>[4x]MATNGMRPIHPGEILRDEFLMEFDISPAALARALKV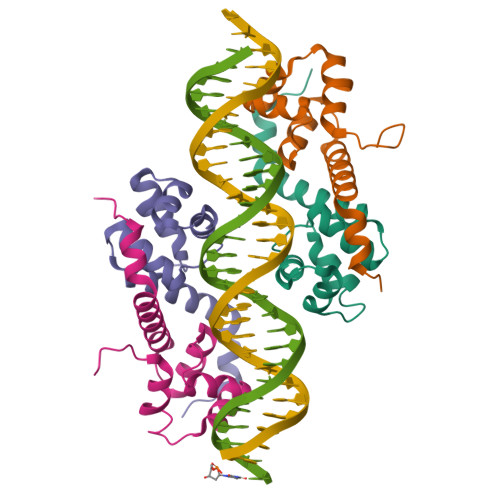SAPTVNDIVREQRGISADMAIRLGRYFDTSAQFWMNLQSEYSLATAYAANGKQIEHEIEPLLAHG> MAQSMYPNEPIVVVGSGCRFPGDANTPSKLWELLQHPRDVQSRIPKERFDVDTFYHPDGKHHGRTNAPYAYVLQDDLGAFDAAFFNIQAGEAESMDPQHRLLLETVYEAVTNAGMRIQDLQGTSTAVYVGVMTHDYETVSTRDLESIPTYSATGVAVSVASNRISYFFDWHGPSMTIDTACSSSLVAVHLAVQQLRTGQSSMAIAAGANLILGPMTFVLESKLSMLSPSGRSRMWDAGADGYARGEAVCSVVLKTLSQALRDGDTIECVIRETGVNQDGRTTGITMPNHSAQEALIKATYAQAGLDITKAEDRCQFFEAHGTGTPAGDPQEAEAIATAFFGHEQVARSDGNERAPLFVGSAKTVVGHTEGTAGLAGLMKASFAVRHGVIPPNLLFDKISPRVAPFYKNLRIPTEATQWPALPPGQPRRASVNSFGFGGTNAHAIIEEYMEPEQNQLRVSNNEDCPPMTGVLSLPLVLSAKSQRSLKIMMEEMLQFLQSHPEIHLHDLTWSLLRKRSVLPFRRAIVGHSHETIRRALEDAIEDGIVSSDFTTEVRGQPSVLGIFTGQGAQWPGMLKNLIEASPYVRNIVRELDDSLQSLPEKYRPSWTLLDQFMLEGEASNVQYATFSQPLCCAVQIVLVRLLEAARIRFTAVVGHSSGEIACAFAAGLISASLAIRIAYLRGVVSAGGARGTPGAMLAAGMSFEEAQEICELDAFEGRICVAASNSPDSVTFSGDANAIDHLKGMLEDESTFARLLKVDTAYHSHHMLPCADPYMQALEECGCAVADAGSPAGSVPWYSSVDAENRQMAARDVTAKYWKDNLVSPVLFSHAVQRAVVTHKALDIGIEVGCHPALKSPCVATIKDVLSGVDLAYTGCLERGKNDLDSFSRALAYLWERFGASSFDADEFMRAVAPDRPCMSVSKLLPAYPWDRSRRYWVESRATRHHLRGPKPHLLLGKLSEYSTPLSFQWLNFVRPRDIEWLDGHALQGQTVFPAAGYIVMAMEAALMIAGTHAKQVKLLEILDMSIDKAVIFDDEDSLVELNLTADVSRNAGEAGSMTISFKIDSCLSKEGNLSLSAKGQLALTIEDVNPRTTSASDQHHLPPPEEEHPHMNRVNINAFYHELGLMGYNYSKDFRRLHNMQRADLRASGTLDFIPLMDEGNGCPLLLHPASLDVAFQTVIGAYSSPGDRRLRCLYVPTHVDRITLVPSLCLATAESGCEKVAFNTINTYDKGDYLSGDIVVFDAEQTTLFQVENITFKPFSPPDASTDHAMFARWSWGPLTPDSLLDNPEYWATAQDKEAIPIIERIVYFYIRSFLSQLTLEERQQAAFHLQKQIEWLEQVLASA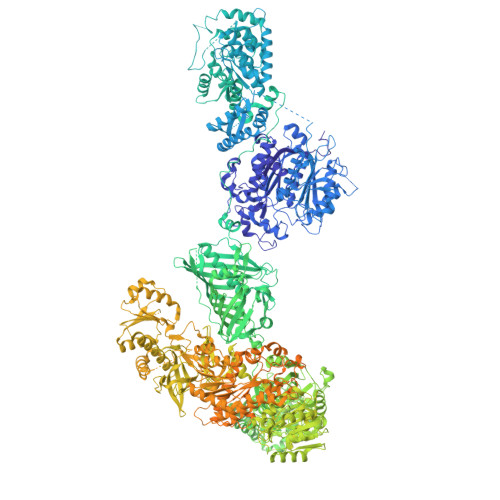KEGRHLWYDPGWENDTEAQIEHLCTANSYHPHVRLVQRVGQHLLPTVRSNGNPFDLLDHDGLLTEFYTNTLSFGPALHYARELVAQIAHRYQSMDILEIGAGTGGATKYVLATPQLGFNSYTYTDISTGFFEQAREQFAPFEDRMVFEPLDIRRSPAEQGFEPHAYDLIIASNVLHATPDLEKTMAHARSLLKPGGQMVILEITHKEHTRLGFIFGLFADWWAGVDDGRCTEPFVSFDRWDAILKRVGFSGVDSRTTDRDANLFPTSVFSTHAIDATVEYLDAPLASSGTVKDSYPPLVVVGGQTPQSQRLLNDIKAIMPPRPLQTYKRLVDLLDAEELPMKSTFVMLTELDEELFAGLTEETFEATKLLLTYASNTVWLTENAWVQHPHQASTIGMLRSIRREHPDLGVHVLDVDAVETFDATFLVEQVLRLEEHTDELASSTTWTQEPEVSWCKGRPWIPRLKRDLARNNRMNSSRRPIYEMIDSSRAPVALQTARDSSSYFLESAETWFVPESVQQMETKTIYVHFSCPHALRVQALGFFYLVQGHVQEGNREVPVVALAERNASIVHVRPDYIYTEADNNLSEGGGSLMVTVLAAAVLAETVISTAKCLGVTDSILVLNPPSICGQMLLHAGEEIGLQVHLATTSGNRSSVSAGDAKSWLTLHARDTDWHLRRVLPRGVQALVDLSADQSCEGLTQRMMKVLMPGCAHYRAADLFTDTVSTELHSGSRHQASLPAAYWEHVVSLARQGLPSVSEGWEVMPCTQFAAHADKTRPDLSTVISWPRESDEATLPTRVRSIDAETLFAADKTYLLVGLTGDLGRSLGRWMVQHGACHIVLTSRNPQVNPKWLAHVEELGGRVTVLSMDVTSQNSVEAGLAKLKDLHLPPVGGIAFGPLVLQDVMLNNMELPMMEMVLNPKVEGVRILHEKFSDPTSSNPLDFFVMFSSIVAVMGNPGQANYSAANCYLQALAQQRVASGLAASTIDIGAVYGVGFVTRAELEEDFNAIRFMFDSVEEHELHTLFAEAVVAGRRAVHQQEQQRKFATVLDMADLELTTGIPPLDPALKDRITFFDDPRIGNLKIPEYRGAKAGEGAAGSKGSVKEQLLQATNLDQVRQIVIDGLSAKLQVTLQIPDGESVHPTIPLIDQGVDSLGAVTVGTWFSKQLYLDLPLLKVLGGASITDLANEAAARLPPSSIPLVAATDGGAESTDNTSENEVSGREDTDLSAAATITEPSSADEDDTEPGDEDVPRSHHPLSLGQEYSWRIQQGAEDPTVFNNTIGMFMKGSIDLKRLYKALRAVLRRHEIFRTGFANVDENGMAQLVFGQTKNKVQTIQVSDRAGAEEGYRQLVQTRYNPAAGDTLRLVDFFWGQDDHLLVVAYHRLVGDGSTTENIFVEAGQLYDGTSLSPHVPQFADLAARQRAMLEDGRMEEDLAYWKKMHYRPSSIPVLPLMRPLVGNSSRSDTPNFQHCGPWQQHEAVARLDPMVAFRIKERSRKHKATPMQFYLAAYQVLLARLTDSTDLTVGLADTNRATVDEMAAMGFFANLLPLRFRDFRPHITFGEHLIATRDLVREALQHARVPYGVLLDQLGLEVPVPTSNQPAPLFQAVFDYKQGQAESGTIGGAKITEVIATRERTPYDVVLEMSDDPTKDPLLTAKLQSSRYEAHHPQAFLESYMSLLSMFSMNPALKLAHVHHHHHH> MIITDVEVRVFRTTTRRHSDSAGHAHPGPAHQVEQAMLTVRTEDGQEGHSFTAPEIVRPHVIEKFVKKVLIGEDHRDRERLWQDLAHWQRGSAAQLTDRTLAVVDCALWDLA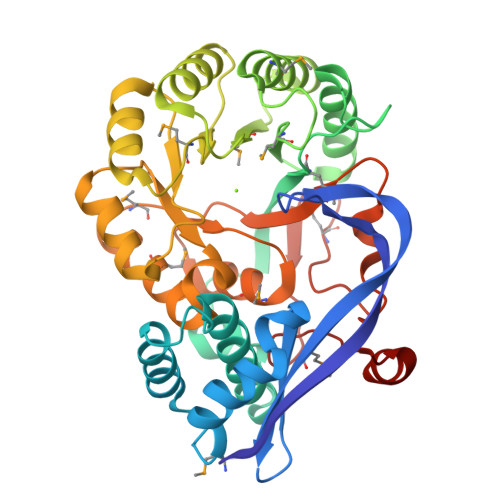GRSLGQPVYKLIGGYRDKVLAYGSIMCGDELEGGLATPEDYGRFAETLVKRGYKGIKLHTWMPPVSWAPDVKMDLKACAAVREAVGPDIRLMIDAFHWYSRTDALALGRGLEKLGFDWIEEPMDEQSLSSYKWLSDNLDIPVVGPESAAGKHWHRAEWIKAGACDILRTGVNDVGGITPALKTMHLAEAFGMECEVHGNTAMNLHVVAATKNCRWYERGLLHPFLEYDDGHDYLKSLSDPMDRDGFVHVPDRPGLGEDIDFTFIDNNRVR> GPMDFVETNSAVYFYGQRDRKFGFLSNFYPCEFTDTEGRRFYSSEQYFMKRKQEMFDRDNEKVAIAILRAKAPAVAKKLGRQVENYDDEVWAEHRYEVMLEALKLKFSSDEEMAAKLLATGAKRLYEASRHDAIWGIGLSVASVTRMFRESVSFQRTGDVDAETRSLCFGKNLLG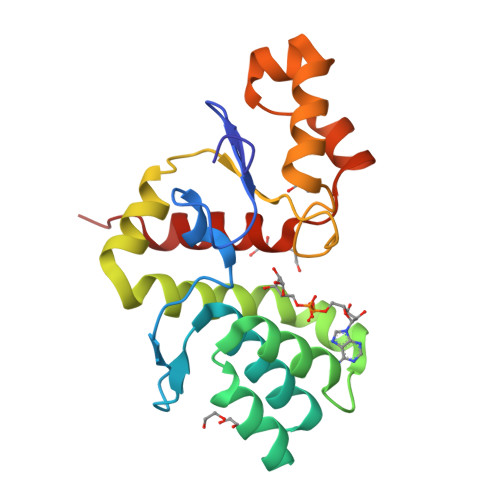NALMEARAWLQPQD N-methyl-N-{2-[({2-[(2-oxo-2,3-dihydro-1H-indol-5-yl)amino]-5-(trifluoromethyl)pyrimidin-4-yl}amino)methyl]phenyl}methanesulfonamide | C22 H21 F3 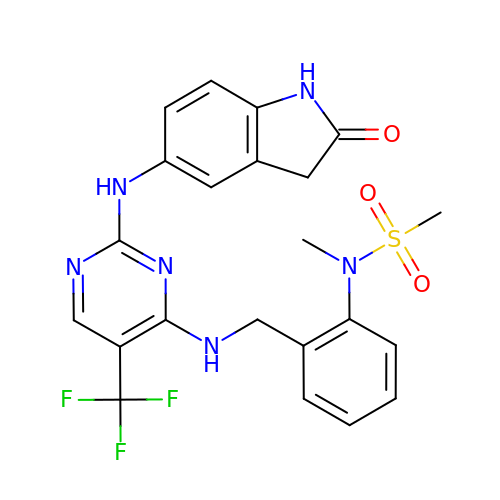N6 O3 S | POJZIZBONPAWIV-UHFFFAOYSA-N> GPGKEDRILKVWTVDPLVKVFRDSEPVTTGQALAEVARGERATLQIVIRCAKPIQELHAK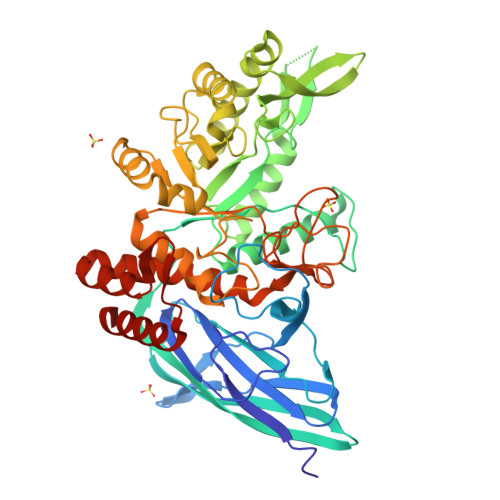VGPLALGSNAKQVLESAPVRFVGYVPVDRPIPRPPKDQLRRPPADFPDPLLEEKTIAVDENQVQPIWVTVAVPTNTQPGLYQGSVHISGRVDGRQITTKVPVAIKVFDIEVGQSRLWVTNWFSMQSRHMKIAPEPDSQQYWALLSRYARNMSEHRQNVVLVSPLSLATFQLDKSSRMEVDFSRFDRWVRIFIAEGVIGRIEGGHLGGRSSDWESPFVVRIKELREGNIITKSVAPTSEEANQFYAQFLPALVNHLRDRGWLEKYAQHLADEPVRTNIESYRAISKLVRKYAPELKIIEACHTKDLAGAIDVWVPQLNFLHNDFEHYQKRQRAGDEVWFYTCIYPQGEYANRFIEQPLLKTRLLHWINYRYGMTGYLHWGYNQWGKDSPFTHTTKQHTGQQYLPAGDPWIVYPGRDGPLDSIRHEAMCDGIADYELLSMLGERDPEAAKRLVNRHVLDFDRYNCNVEAFRATRLELLELLSRQ7-{2-[(3-fluorobenzyl)amino]ethyl}quinolin-2-amine | C18 H18 F N3 | 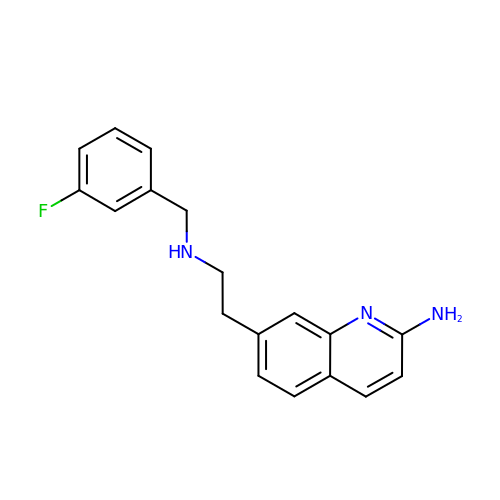GFTZBOUXJJDHLM-UHFFFAOYSA-N STIGMATELLIN | C30 H42 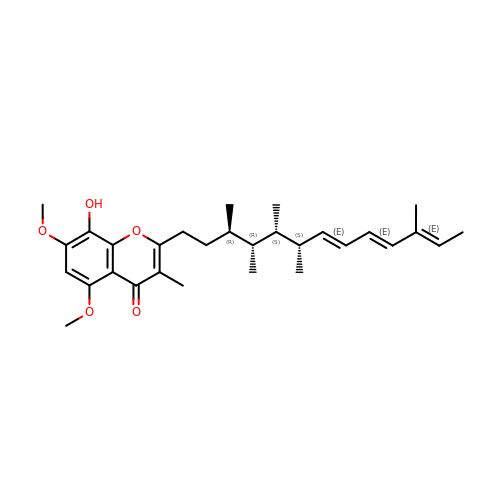O5 | UDPIGEIYWVCFED-RBWCRZADSA-N> MEPIIRIRNLHKWFGPLHVLKGIHLEVAPGEKLVIIGPSGSGKSTLIRTINRLEDFQEGEVVVDGLSVKDDRALRE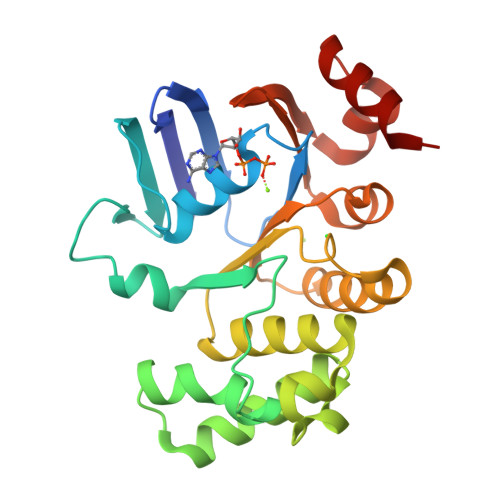IRREVGMVFQQFNLFPHMTVLENVTLAPMRVRRWPREKAEKKALELLERVGILDQARKYPAQLSGGQQQRVAIARALAMEPKIMLFDEPTSALDPEMVGEVLDVMRDLAQGGMTMVVVTHEMGFAREVADRVVFMDGGQIVEEGRPEEIFTRPKEERTRSFLQRVLHH>[2x]SPYSSDTTPCCFAYIARPLPRAHIKEYFYTSGK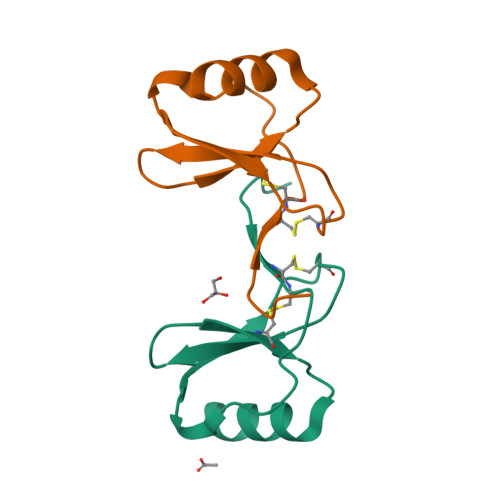CSNPAVVFVTRKNRQVCANPEKKWVREYINSLSMS2-{2-[(cyclopropanesulfonyl)amino]-1,3-thiazol-4-yl}-2-methyl-N-{5-[6-(trifluoromethyl)pyrazin-2-yl]pyridin-2-yl}propanamide | C20 H19 F3 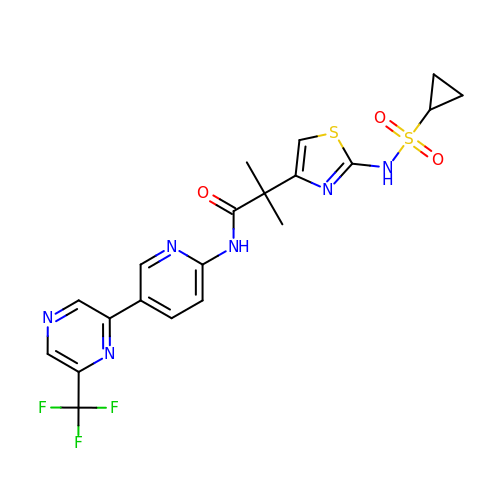N6 O3 S2 | CZIDGRDZSFIUHX-UHFFFAOYSA-N> AAWKWWEEERYPEGIKWKFLEHKGPVFAPPYEPLPENVKFYYDGKVMKLSPKAEEVATFFAKMLDHEYTTKEIFRKNFFKDWRKEMTNEEKNIITNLSKCDFTQMSQYFKAQTEARKQMSKEEKLKIKEENEKLLKEYGFCIMDNHKERIANFKIEPPGLSRGRGNHPKMGMLKRRIMPEDIIINCSKDAKVPSPPPGHKWKEVRHDNKVTWLVSWTENIQGSIKYIMLNPSSRIKGEKDWQKYETARRLKKCVDKIRNQYREDWKSKEMKVRQRAVALYFIDKLALRAGNEKEEGETADTVGCCSLRVEHINLHPELDGQEYVVEFDF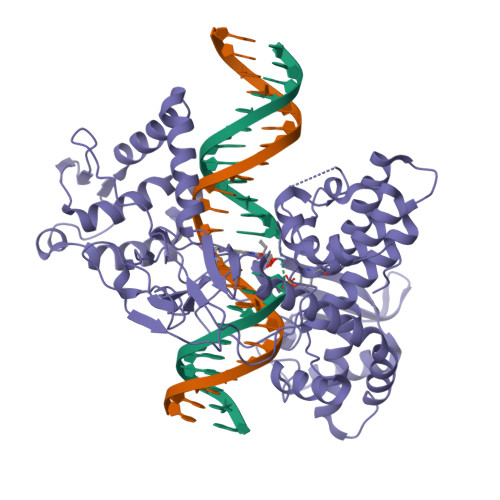LGKDSIRYYNKVPVEKRVFKNLQLFMENKQPEDDLFDRLNTGILNKHLQDLMEGLTAKVFRTYNASITLQQQLKELTAPDENIPAKILSYNRANRAVAILCNHQQAPPKTFEKSMMNLQTKIDAKKEQLADARRDLKSAKADAKVMKDAKTKKVVESKKKAVQRLEEQLMKLEVQATDREENKQIALGTSKLNYLDPRITVAWCKKWGVPIEKIYNKTQREKFAWAIDMADEDYEF> MIGEKDIQPILKNLQRFEGVRGVIITTTEGLPISTTIDREKTEKTAALVTSLVGKARSTVKELEEGELKFLTINTSKGE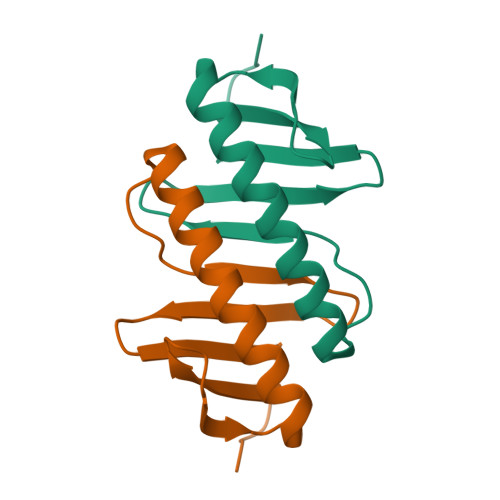VHVAQEEDYILIVLK>GHMSDKRNPRISSRKQPQQARSSELVASILEAAVQVLASEGAQRFTTARVAERAGVSIGSLYQYFPNKAAILFRLQSDEWRRTTRLLGEILEDTTRPPLERLRRLVLAFVRSECEEAAIRVALSDAAPLYRDADEAREVKAEGARVFQAFLREALPEVAEAERSLAGDLLTTTLGAVGKQFSEQPRSEAEIERYAEALADMLCAYL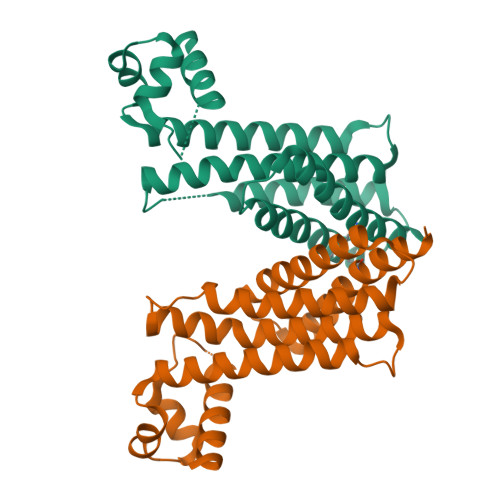AALGERGS[2x]>[2x]GHMAIATINPTTGEICQRFKALTPAEIDAKLAKAQEAFQAYRRTSFSQRRQWLENAAAILERDTSKFAEIMTTEMGKTHQSAIAEAEKSALVCRYYAEHGEQFLANEYTETQATESYVCYQPLGILLAVMPW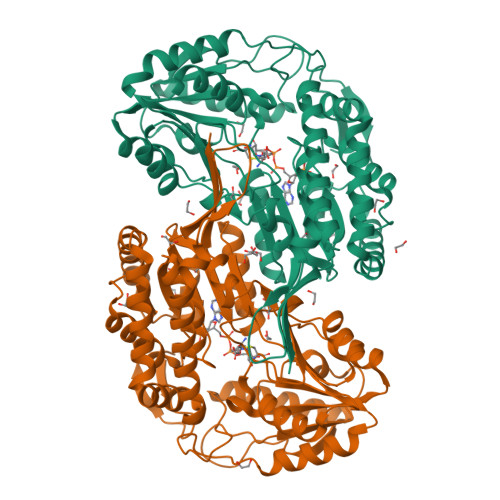NFPFWQVFRFAAPALMAGNVAVLKHASNVPQCALAVEAILEAAGFPEGVFQTLLIGASQVEQVIKDPRVKAATLTGSEPAGASLASLAGQEIKPTLLELGGSDPFVVFPSADLDEAVEVGTVARTMNNGQSCIAAKRFILHEAIAAEFLEKLHLKFASLKIGDPMAPETDIGPLATEGILQDISRQVDQAVAAGAKILLGGRPLDRAGYFYPPTILTEIPPGAKILQEELFAPVAMVFTVKDLDQAIALANDIPFGLGASAWTNDPAEQQRFIQELDAGAVFINGMVKSDPRLPFGGTKRSGYGRELGLAGIRTFVNAKTVWLK During exocytosis, a protein complex called the exocyst mediates the tethering of vesicles to the plasma membrane. The exocyst is an octamer formed by the proteins Sec3, Sec5, Sec6, Sec8, Sec10, Sec15, Exo70, and Exo84 (3), which assemble in a holocomplex to control the spatiotemporal regulation of exocytosis, orchestrate cargo delivery, and mediate vesicle secretion. One such effector, AVR-Pii, interacts with two rice Exo70 subunits, OsExo70F2 and OsExo70F3, suggesting that the pathogen may target exocyst-mediated trafficking as a virulence-associated mechanism. Here, we reveal the structural basis of how an effector from the blast pathogen (AVR-Pii) binds a specific host target (rice Exo70) and how this underpins immune recognition.

Using this sample, we obtained protein crystals that diffracted X-rays to 2.7 Å resolution at the Diamond Light Source (Oxford, United Kingdom). In the crystal structure, AVR-Pii and OsExo70F2 form a 1:1 complex. OsExo70F2 adopts an elongated rod-like shape formed by the stacking of four domains (domains A to D), with 16 α-helices in total (annotated α1 to α16) arranged in four-helix bundles. Following placement of OsExo70F2, we identified an electron density consistent with the sequence of AVR-Pii and were able to build residues 44 to 70 of the effector (residues 20 to 43 were not observed in the electron density). A structural similarity search performed with PDBeFold revealed the AVR-Pii structure is most similar to LIM domain zinc fingers with a motif of C-X2-C-X12-H-X-C; however, it lacks a second zinc binding motif commonly found in this class of domains. We refer to the AVR-Pii fold as ZiF and note that this three-dimensional structure has not been previously reported to our knowledge for other plant pathogen effectors and is distinct from the MAX fold found for other M. oryzae effectors whose structures are known. AVR-Pii locates to an amphipathic surface formed at the junction of OsExo70F2 domains B and C, with residues from helices α8, α9, and α10 contributing to the effector binding interface. Analysis of the complex using QtPISA reveals both hydrophobic and hydrogen bond interactions in the complex, with a remarkable 20 of the 27 AVR-Pii residues (74%) observed for the effector in the crystal structure involved in contacts with OsExo70F2. The most striking feature of the OsExo70F2/AVR-Pii interface is a hydrophobic pocket formed by OsExo70F2 residues Phe416, Leu420, Met437, Tyr440, and Val441, which accommodates AVR-Pii Phe65 and, to a lesser extent, Tyr64.

> ISAAAFDAAEQLIQVWDGTPEALVFEATEDEVAEYLSAVDVAIEHLARGSGGGAGGAGSSSSSTAGRAGVAVQLAMARLEEELRHLMVRHAVPLDPTGLFFSLRRLSLGSMDDLDTSSEFDAATPHSIDVAPETARGGPLVNPFEDQVFDPVRPEAVDDLRAIADRMARAGYSRELADAYCGIRRDLLDEYLSALGVERLSIDEVQRIEWKHLNDKMKKWVQAVKTVVRVLLAGERRLCDQVLSVSDELREECFIESTKGCIMQILSFGDAVAVCPRSPEKLSRILDMYEALAEVIPEMKDLCLGSSGDGVISDVQANLDRLGDAIRGTLFEFGKVLQLESSRRAMTAGEIHPMTRYVMNYLRLLVVYSDTLDALLDDNADDQIDLARAEDQDQEHLESMTPLGKRLLKLISYLEANLEEKSKLYEDSALECIFSMNNLLYIVQKVRDSELGKILGDHWVKRRNGKIRQYSKSYLRISWMKVLSFLKDDGHGSGSGSSSGSGSGHSSSRMSIKEKFKNFNLAFEEIYRNQTTWKVPDPQLREELKISISENVIPAYRAFLGRYGSQVDGGRNSGKYIKYTPEDLESQLSDLFEGAPGPANHSRRRT;> LPTPASLNGNTEVATISDVKLEARSDTTYHKCSKCGYGSDDSDAYFNHKCN> SQNGRIDPFTLVLGPLYAIDAPFAVNLVSQNGRRYLKASISLELSNEKLLNEVKVKDTAIKDTIIEILSSKSVEEVVTN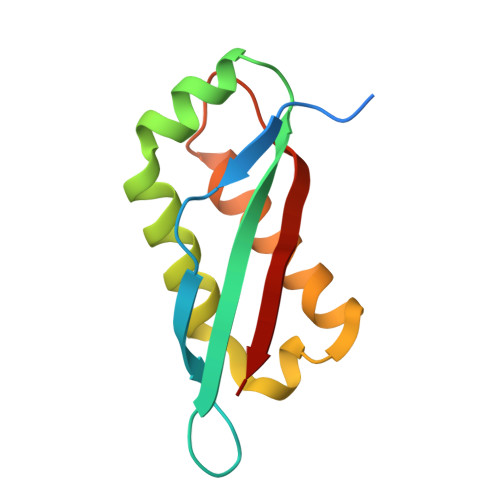KGKNKLKDEIKSHLNSFLIDGFIKNVFFTDFIIQ>GGNSFVGL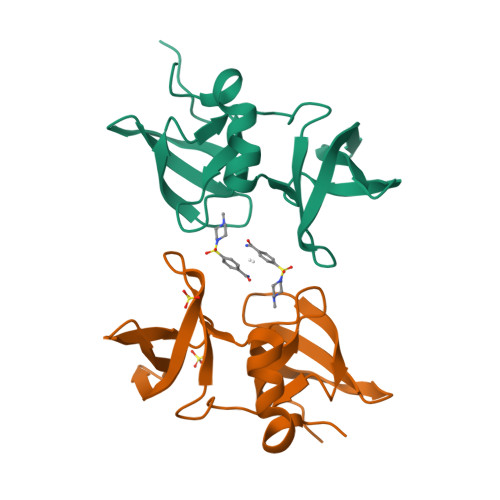RVVAKWSSNGYFYSGKITRDVGAGKYKLLFDDGYECDVLGKDILLCDPIPLDTEVTALSEDEYFSAGVVKGHRKESGELYYSIEKEGQRKWYKRMAVILSLEQGNRLREQYGLGPYE[2x]> H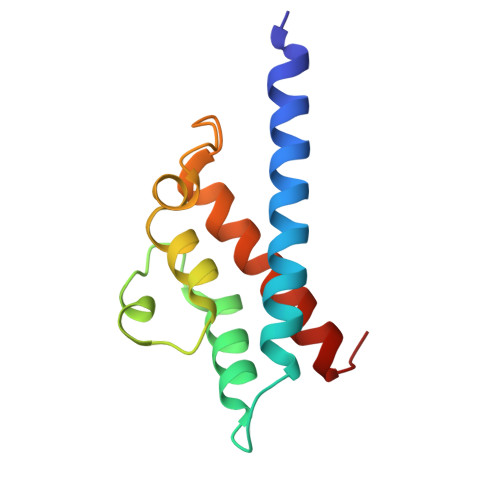MFFKDYQKKNVMRLLQDSLEKIINEWLKTDDESHTKLKSLQELSEMDINATSFAEHSPLPDFVTRLWLDPHKALDAMDKNISKNEIRKLIKETAREIELVFTHQK(2Z,6Z)-3,7,11-trimethyldodeca-2,6,10-trien-1-yl 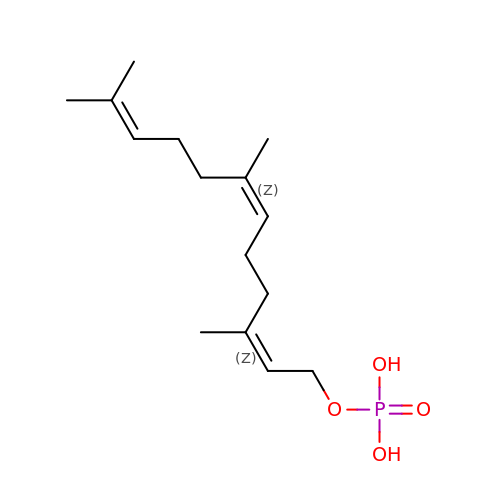dihydrogen phosphate | C15 H27 O4 P | ALEWCKXBHSDCCT-FBXUGWQNSA-N> PGNSTGSNATNNTTNTTPTPTPSGSVNGAAIVAEAYKYIGTPYVWGGKDPSGFDCSGFTRYVYLQVTGRDIGGWTVPQESAGTKISVSQAKAGDLLFWGSPGGTYHVAIALGGGQYIHAPQPGESVKVGSVQWFAPDFAVSMLEHHHHHH

The protective activity of E. faecium growth media was protease sensitive, which led to the proteomic analysis of the supernatant and discovery of secreted antigen A (SagA) as one of the most abundant E. faecium secreted proteins. SagA encodes an N-terminal signal sequence, predicted coiled-coil domain, Ser/Thr-rich linker region and C-terminal NlpC/p60-family peptidase domain. The identity of GlcNAc-MDP was further confirmed by LC-MS/MS analysis and its fragmentation into MDP. These results demonstrated that SagA-NlpC/p60 encodes cysteine endopeptidase activity that prefers crosslinked peptidoglycan fragments and cleaves the peptide bond between D-iGln and L-Lys. Collectively, our results suggest that E. faecium and its secreted peptidoglycan hydrolase SagA generates small muropeptides that activate NOD2, which triggers downstream signaling pathways to enhance intestinal barrier function and host immunity.

To understand the molecular mechanism of E. facium SagA-NlpC/p60, we determined crystal structure of the E. faecium SagA-NlpC/p60 domain. Gel-filtration analysis revealed that SagA-NlpC/p60 is monomeric and amenable to crystallization (Supplementary Results). The structure of the SagA-NlpC/p60 domain was solved to 2.4 Å resolution by using X-ray crystallography. The SagA-NlpC/p60 domain contained the typical features of the cysteine peptidase fold, a central six-stranded, antiparallel β-sheet flanked by three surrounding α-helices. The overall dimensions of the structure were about 32.5 × 30×23 Å and shared significant structural homology to other NlpC/p60 hydrolase domains. The root-mean-square deviations between superimposed Cα atoms was a range of 1.6 ~ 2.0 Å when comparing with NlpC/p60 hydrolase domains of other structures. The conserved catalytic triad (C443, H494 and H506) of the SagA-NlpC/p60 domain was located in a putative substrate-binding groove between the subdomains in the α2 and β3–β4, where electron density for these key amino acid residues were well observed. An electrostatic potential analysis of the SagA-NlpC/p60 domain showed that the putative substrate-binding groove was mostly composed of negatively charged amino acid residues. Structural alignments with other homologs also showed similar conformations of the catalytic triad in the active site to that of the YkfC from Bacillus cereus, NpPCP from Nostoc punctiforme, AvPCP from Anabaena variabilis, CwlT from Staphylococcus aureus, Spr from Escherichia coli, RipA from Mycobacterium tuberculosis, and LysM from Thermus thermophilus active sites. Indeed, single and double Ala mutants of W433 and W462 significantly abrogated hydrolytic activity of SagA-NlpC/p60 domain. These results demonstrate C443, W433 and W462 are crucial for the SagA-NlpC/p60 peptidoglycan hydrolase activity and encompass the enzyme active site as well as putative substrate-binding groove.> ASGFNAAEDAQTLRKAMKGLGTDEDAIINVLAYRSTAQRQEIRTAYKTTIGRDLMDDLKSELSGNFEQVILGMMTPTVLYDVQEVRKAMKGAGTDEGCLIEILASRTPEEIRRINQTYQLQYGRSLE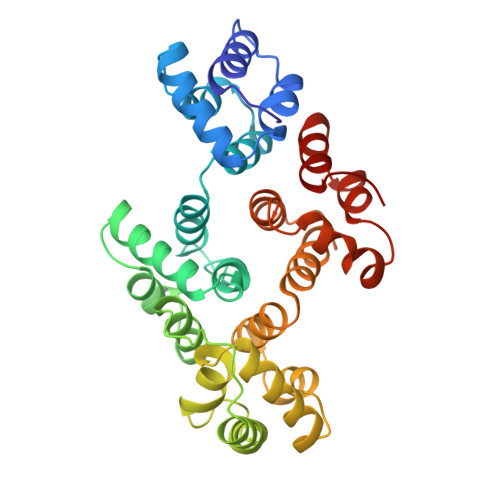DDIRSDTSFMFQRVLVSLSAGGRDESNYLDDALMRQDAQDLYEAGEKKWGTDEVKFLTVLCSRNRNHLLHVFDEYKRIAQKDIEQSIKSETSGSFEDALLAIVKCMRNKSAYFAERLYKSMKGLGTDDDTLIRVMVSRAEIDMLDIRANFKRLYGKSLYSFIKGDTSGDYRKVLLILCGGDD>MASVHGTTYELLRRQGIDTVFGNPGSNELPFLKDFPEDFRYILALQEACVVGIADGYAQASRKPAFINLHSAAGTGNAMGALSNAWNSHSPLIVTAGQQTRAMIGVEALLTNVDAANLPRPLVKWSYEPASAAEVPHAMSRAIHMASMAPQGPVYLSVPYDDWDKDADPQSHHLFDRHVSSSVRLNDQDLDILVKALNSASNPAIVLGPDVDAANANADCVMLAERLKAPVWVAPSAPRCPFPTRHPCFRGLMPAGIAAISQLLEGHDVVLVIGAPVFRYHQYDPGQYLKPGTRLISVTCDPLEAARAPMGDAIVADIGAMASALANLVEESSRQLPTAAPEPAKVDQDAGRLHPETVFDTLNDMAPENAIYLNESTSTTAQMWQRLNMRNPGSY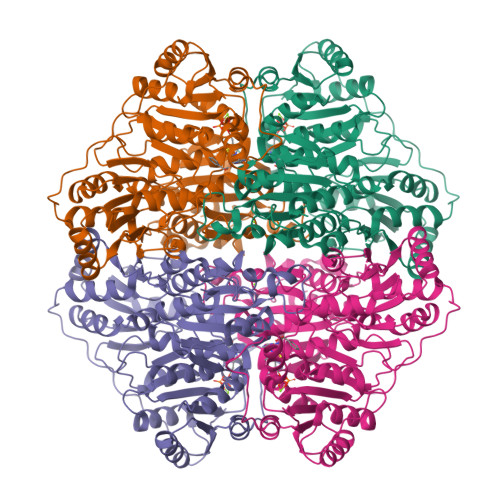YFCAAGGLGFALPAAIGVQLAEPERQVIAVIGDGSANYSISALWTAAQYNIPTIFVIMNNGTYGALRWFAGVLEAENVPGLDVPGIDFRALAKGYGVQALKADNLEQLKGSLQEALSAKGPVLIEVSTVSPVK[16x]>XGEIAQALKEIAQALKESAKATKESAWATKEIAQAL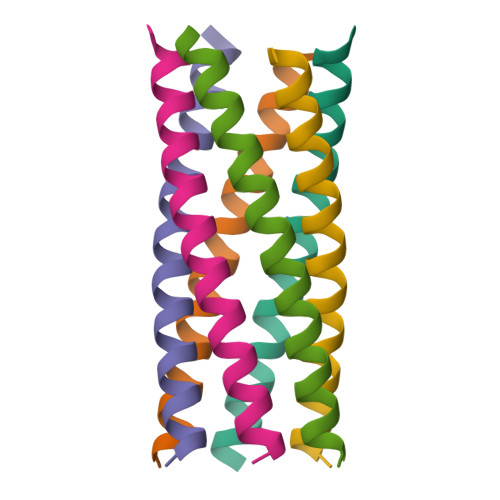KGX[12x]>SKRNKPGKATGKGKPVNNKWLNNAGKDLGSPVPDRIANKLRDKEFKSFQDFRKKFWEEVSKDPEL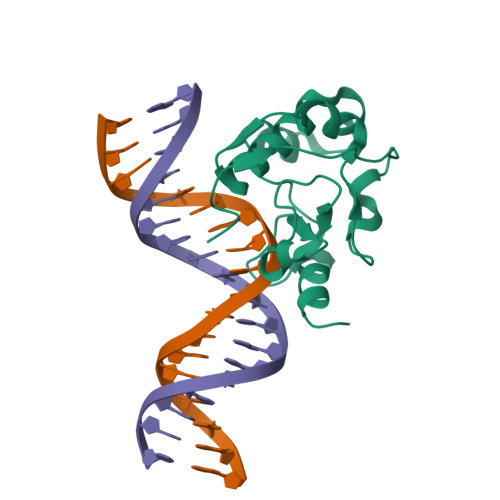SKQFSRNNNDRMKVGKAPKTRTQDVSGKRTSFELHHEKPISQNGGVYDMDNISVVTPKRHIDIHRGK[2x]>GSAKDPMHNFTYWNPTKLIFGRGEVERLPEELKSYGKNVLLVYGGGSIKRSGLYDQVIEQLNKAGVTVHELAGVEPNPRVSTVNKGVALCKEHHIDFLLAVGGGSVIDCTKAIAAGAKYDGDAWDIVTKKHQPKDALPFGTVLTLAATGSEMNSGSVITNWETKEKYGWGSPLVFPKFSILDPVNTFTVPKNHTIYGMVDMMSHVFEQYFHHVSNTPYQDRMCESLLRTVIETAPKLINDLENYELRETILYTGTIALNGMLSMGARGDWATHNIEHAVSAVYDIPHAGGLAILFPNWMRHTLSENPARMKQLAVRVFGVEEAGKTDKEVALEGIDKLSAFWTSLGAPNRLADYDINDEQLDTIADKAMANGTFGQFKSLNKEDVLAILKASL[4x]

Based on structural and biochemical studies, we report here that YugJ from B. subtilis is an atypical NADPH-dependent group III AAOR that reduces furan aldehyde in the presence of a Ni2+ cofactor. YugJ folds into a two-domain structure consisting of a Rossmann-like domain and an α-helical domain. YugJ interacts with NADP and Ni2+ using the interdomain cleft of YugJ. YugJ was highly active as an HMF reductase when supplemented with NADPH, but it was inactive with NADH, indicating that YugJ is an NADPH-dependent aldehyde reductase.

To address the specific interaction of YugJ with NADP(H), we determined the crystal structures of YugJ in complex with NADP in two crystal forms. The first crystal structure (space group P1) contains both the NADP cofactor and Ni2+ ion and was named YugJNADP-Ni. However, in the YugJNADP-Ni structure, the nicotinamide ring of NADP is disordered, and only the remaining NADP region was built. However, in the YugJNADP-Ni structure, the nicotinamide-YugJ interaction is not observed because of nicotinamide disorder. On the other hand, in the nitrate-less YugJNADP-Ni structure, the nicotinamide ring of NADP is disordered, although similar conformations are observed for the YugJ Asp102, Asn147, and Gly149 residues that interact with nicotinamide in the YugJNADP-NO3 structure. Thus, we propose that NADP(H) nicotinamide in YugJ prefers high structural dynamics for substrate recognition and becomes rigid upon substrate binding. Each protomer of the NADP-bound YugJ structures (YugJNADP-Ni chains A, B, C, and D and YugJNADP-NO3 chains A and B) adopts a closed conformation with a smaller interdomain angle, similar to that of YugJNi chain B. However, NADP binding restricts the interdomain organization of YugJ into the closed conformation. In contrast, the α9–α10 loop of the YugJNi and YugJNADP-Ni structures adopts an open conformation that increases the accessibly of the active site. Accordingly, an additional three-pointed density was not observed in the YugJNi or YugJNADP-Ni structure obtained in the absence of nitrate.>[2x]GMDKLNEYRTKVRQLLTKHLQYKPSYGDVEV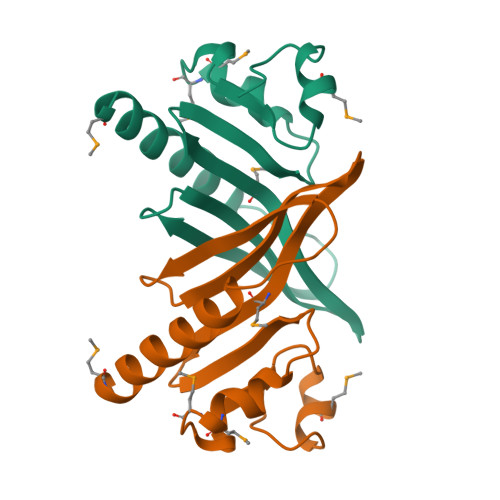EQIFDEEHDHYQIISVGWNNQHRIYGPIMHLDIKNNKIWIQQNTTEADIALELMEMGIDKQDIVIGFHTPKMRQLSGFAVE The AP–NHEJ repair complex is primarily composed of a Ku homodimer, DNA ligase (Lig), DNA polymerase (Pol) and a phosphoesterase (PE). Studies on NHEJ repair in Mtu and the archaeon Methanocella paludicola (Mpa) demonstrated that both species possess equivalent core AP–NHEJ components, with orthologous proteins possessing near identical substrate specificities. We discovered that Pol has DNA strand displacement activity during RNA synthesis and that PE resects excessive incorporation to promote efficient break ligation. In this current study, we sought to extend our understanding of AP–NHEJ by comparing crystal structures of the archaeal (Mpa) Pol and PE with those of the established bacterial (M. tuberculosis and P. aeruginosa) DSB repair complexes.

We previously reported that the M. paludicola phosphoesterase (Mpa PE), which is operonic with an NHEJ RNA/DNA primase–polymerase and ligase, is a functional component of the archaeal NHEJ repair apparatus. To understand more about the molecular mechanism of these atypical nucleases, we elucidated the crystal structure of Mpa PE at a resolution of 1.79 Å. A ribbon diagram of the PE protein shows a hydrophobic core formed of a β-barrel super secondary structure, composed of nine anti-parallel strands. The β-barrel is surrounded by four α-helices and a 310 helix, as observed in a prokaryotic PE structure. The exterior of the β-barrel provides a cavity for the active site, which is enclosed by the 310 helix and a surface loop. A surface representation of Mpa PE is shown in Figure 1B and C, in which vanadate and magnesium ions can be observed occupying a cleft. Since vanadate is a structural analogue for phosphate, we infer that the vanadate ion is occupying the position of the scissile phosphate, positioned in between the six key catalytic residues: H40, H46, D48, R50, H82 and Y86. We predict that this cleft is a DNA binding channel. Analysis of the crystal structure of Mpa PE suggested that the conserved histidine residue (H82) may be one of the key residues in positioning the scissile phosphate in the active site.

> IKHPIYVIQKHDASHLHYDLRLEMGGVLKSWAVPKGPSLDPKVKRLAMPTEDHPIGYATFEGVIPEGQYGGGTVMVWDIGTYRNLREEKPEGSRMTIEQSYDQGKIEVFLEGKKLKGSYALIRTGGIEKRGWLFFKMKEPHEGSYEDIEKAAPDSVLTGRTMDEIAKEG> GPYMIQEEEWDRDLLLDPAWEKQQRKTFTAWCNSHLRKAGTQIENIEEDFRNGLKLMLLLEVISGERLPKPDRGKMRFHKIANVNKALDYIASKGVKLVSIGA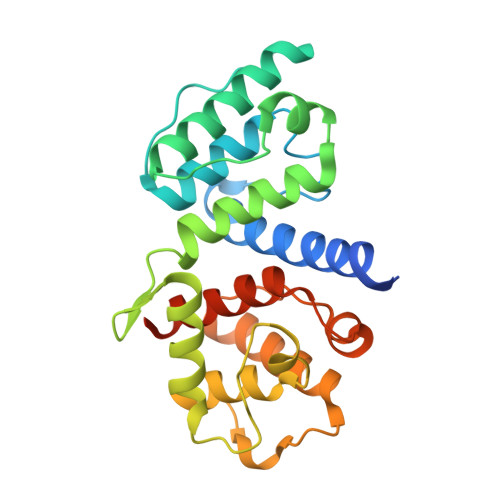EEIVDGNVKMTLGMIWTIILRFAIQDISVEETSAKEGLLLWCQRKTAPYRNVNIQNFHTSWKDGLGLCALIHRHRPDLIDYSKLNKDDPIGNINLAMEIAEKHLDIPKMLDAEDIVNTPKPDERAIMTYVSCFYHAFAGAEQAETAANRIC>[2x]DYKDDDDKMVFEQHEEEAVAPGAVHGHRLSTVVPSSVTGEVDYALADADLAFKLHYLRGVYYYRSGDGLATKVLKDPMFPWLDDHFPVAGRVRRAEAEGDGAPRRPYIKCNDCGVRIVEARCDRDMAEWIRDAAPGRIRQLCYDKVLGPELFFSPLLYVQITNFKCGGLALGFSWAHLIGDIPSAATCFNKWAQILSGKKPEATVLTPPNQPLQGQSPAAPRSVKQVGPMEDLWLVPAGRDMACYSFHVSDAVLKKLHQQQNGRQDAAAGTFELVSALVWQAVAKIRGDVDTVTVVRADAAARSGKSLANEMKVGYVESAGSSPAKTDVAELAALLAKNVVDETAAVAAFQ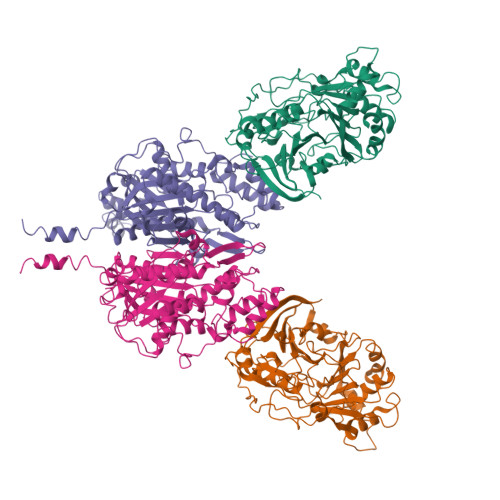GDVLVYGGANLTLVDMEQVDLYGLEIKGQRPVYVEYGMDGVGDEGAVLVQPDADGRGRLVTVVLPGDEIDSLRAALGSALHVA;>HHHHHHMPSGGVFSGSVNLKHVKLGYQYLVNHFLTLLLVPVMAATALELARLGPGELLSLWRSLELDLVHILCSAFLVVFVGTVYVMSRPRPVYLVDYACYKPPASCRVPFATFMEHTRLISDDDKSVRFQTRILERSGLGEDTCLPPANHYIPPNPSMEASRAEAQLVIFSAIDDLVRRTGLKPKDIDILVVNCSLFSPTPSLSAMIINKYKLRSNIRSFNLSGMGCSAGLISIDLARDMLQVHPNSNALVVSTEIITPNFYQGSRRDMLLPNCLFRMGAAAILLSNRRREARRAKYRLVHVVRTHKGADDRAYRCVYEEEDEQGFSGISLSKELMAIAGDALKSNITTIGPLVLPMSEQLLFFFRLVGRKLVNKGWRPYIPDFKLAFEHFCIHAGGRAVIDELQKNLQLSPRHVEASRMTLHRFGNTSSSSLWYELAYIEAKGRMRRGDRVWQIGFGSGFKCNSAVWKCLRSIKTPTNGPWDDCIHRYPVDVPEVVKL[2x]The folate metabolism enzyme MTHFD2 (methylenetetrahydrofolate dehydrogenase/cyclohydrolase) is consistently overexpressed in cancer but its roles are not fully characterized, and current candidate inhibitors have limited potency for clinical development. Indeed, the one-carbon metabolism enzyme MTHFD2 stands out as the most consistently overexpressed metabolic enzyme across human tumors. MTHFD2 enzymatic function supports rapid cell proliferation during early embryogenesis, after which it is replaced by the mitochondrial protein MTHFD2L in healthy mature tissue.

The tool compound TH7299, as well as two of the most promising candidates, TH9028 and TH9619, were chosen to investigate the MTHFD2 mechanism of action and cancer biology. Furthermore, we determined the cocrystal structures of TH7299, TH9028 and TH9619 in complexes with human MTHFD2 to assess their binding mode and identify critical interactions in the binding pocket. In the present study, we show that, in contrast to the characteristic promiscuity and polypharmacology of antifolates such as methotrexate (MTX) and pemetrexed (PMTX), TH9619 displayed high selectivity toward binding and stabilizing MTHFD2 over other common folate metabolism targets such as dihydrofolate reductase (DHFR), thymidylate synthase (TYMS), serine hydroxymethyltransferase (SHMT) 1 and SHMT2. We could confirm MTHFD2 stabilization against thermal degradation on incubation with TH9619 in cell lysates and live cells using CETSA, demonstrating intracellular target engagement. To evaluate whether targeting MTHFD2 was responsible for the observed toxicity on MTHFD2 inhibitors in cancer cells, we generated MTHFD2−/− clustered regularly interspaced short palindromic repeats (CRISPR)–Cas9 knockout cells and found that they were several orders of magnitude more resistant to TH9619 than parental MTHFD2 WT cells, but not MTHFD1−/− cells. TH9619 shows very good solubility and metabolic stability in combination with low plasma protein binding, but also poor passive cell permeability that is probably explained by the low lipophilicity (cLogP: −2.25) and large polar surface area (239 Å2 (23.9 nm)), suggesting active transport over membranes, probably via folate transporters and/or receptors. Furthermore, TH9619 was comparably potent against mouse MTHFD2 (half-maximal inhibitory concentration (IC50) of 66 nM), indicating that mice could be used as a model for safety and tolerability studies.

>MEAVVISGRKLAQQIKQEVRQEVEEWVASGNKRPHLSVILVGENPASHSYVLNKTRAAAVVGINSETIMKPASISEEELLNLINKLNNDDNVDGLLVQLPLPEHIDERRICNAVSPDKDVDGFHVINVGRMCLDQYSMLPATPWGVWEIIKRTGIPTLGKNVVVAGRSKNVGMPIAMLLHTDGAHERPGGDATVTISHRYTPKEQLKKHTILADIVISAAGIPNLITADMIKEGAAVIDVGINRVHDPVTAKPKLVGDVDFEGVRQKAGYITPVPGGVGPMTVAMLMKNTIIAAKKVLRLEEREVLKSKELGVATN[2x]>[3x]IDQKEKELIKESWKRIEPNKNEIGLLFYANLFKEEPTVSVLFQNPISSQSRKLMQVLGILVQGIDN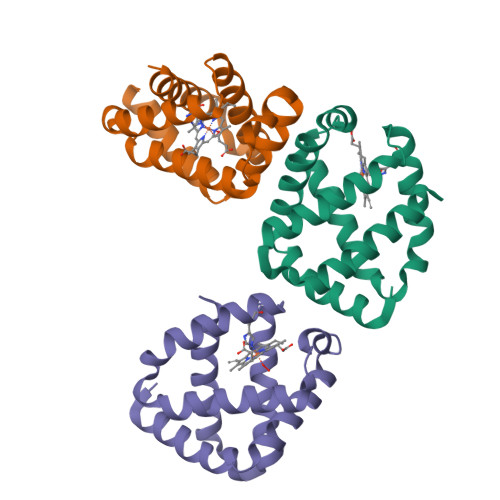LEGLIPTLQDLGRRHKQYGVVDSHYPLVGDCLLKSIQEYLGQGFTEEAKAAWTKVYGIAAQVMTA> MEQANPLRPDGESKGGVLAHLERLETQVSRSRKQSEELQSVQAQEGALGTKIHKLRRLRDELRAVVRHRRASVKACIANVEPNQTVEINEQEALE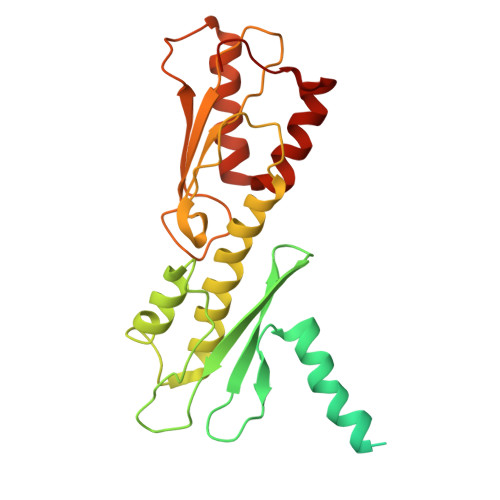EKLENVKAILQAYHFTGLSGKLTSRGVCVCISTAFEGNLLDSYFVDLVIQKPLRIHHHSVPVFIPLEEIAAKYLQTNIQHFLFSLCEYLNAYSGRKYQADRLQSDFAALLTGPLQRNPLCNLLSFTYKLDPGGQSFPFCARLLYKDLTATLPTDVTVTCQGVEVLSTSWEEQRASHETLFCTKPLHQVFASFTRKGEKLDMSLVS>MNLPTAQEVQGLMARSIELVDVGDIEAIVQMYADDATVENPFGQPPIHGREQIAAFYRQGLGGGKVRACLTGPVRASHNGCGAMPFRVEMVWNGQPCALDVIDVMRFDEHGRIQTMQAYWSEVN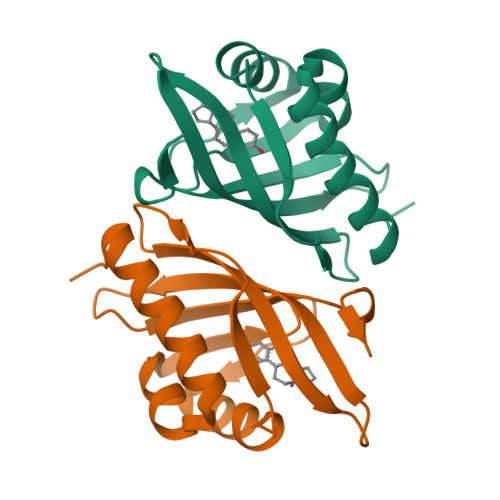LSVREPQ[4x]>SNAKDVLGLTLLEKTLKERLNLKDAIIVSGDSDQSPWVKKEMGRAAVACM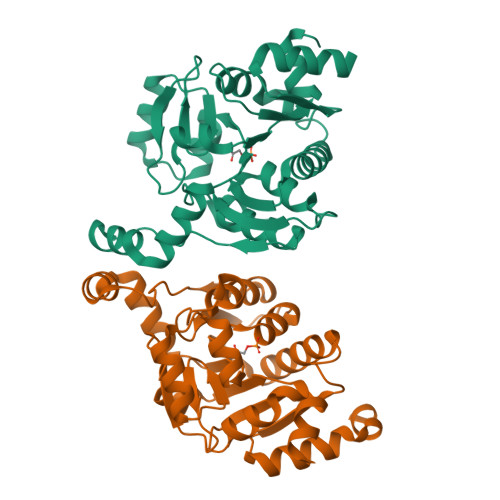KKRFSGKNIVAVTGGTTIEAVAEMMTPDSKNRELLFVPARGGLGEDVKNQANTICAHMAEKASGTYRLLFVPGQLSQGAYSSIIEEPSVKEVLNTIKSASMLVHGIGEAKTMAQRRNTPLEDLKKIDDNDAVTEAFGYYFNADGEVVHKVHSVGMQLDDIDAIPDIIAVAGGSSKAEAIEAYFKKPRNTVLVTDEGAAKKLLRDE[2x]>[3x]MAEIYNKDGNKVDLYGKAVGLHYFSKGNGENSYGGNGDMTYARLGFKGETQINSDLTGYGQWEYNFQ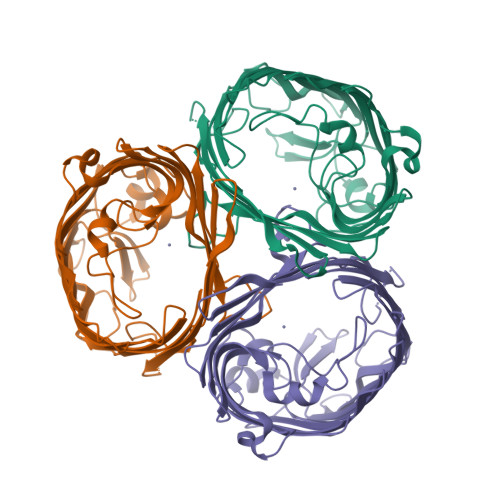GNNSEGADAQTGNKTHLAFAGLKYADVGSFDYGRNHGVVYDALGYTDMLPEFGGDTAYSDDFFVGHVGGVATYRNSNFFGLVDGLNFAVQYLGKNERDTARRSNGDGVGGSISYEYEGFGIVGAYGAADRTNLQEAQPLGNGKKAEQWATGLKYDANNIYLAANYGETRNATPITNKFTNTSGFANKTQDVLLVAQYQFDFGLRPSIAYTKSKAKDVEGIGDVDLVNYFEVGATYYFNKNMSTYVDYIINQIDSDNKLGVGSDDTVAVGIVYQF> MAANEGNQPIPPEEEKEISSLLESIKIGKTSLKYRCFYLYDDKMTDLTEEQKETLKKLKLYQKEYYDYESKFEYELFLLRQKYHDLYGPIYDKRREALVGNGEAKIGTPNLPEFWLRALRNNNTVSHVIEDHDEEILVYLNDIRCDYIKKNKEKKEGFILSFYFATNPFFSNSVLTKTYHMKCVDCDNEPVLLHTEATVIDWYDNKNILKKNVVKKQHNKNSREVKTVQQTVNRDSFFHFFTSHKVPNSNVIKQLSKHEVAQLEMIIEGDYEVALTIKERIIPYAVDYYLGIIIESESNSIVSDVDSSYSSSENNSNYNSYESNNSAYNDENSNVDTNEYDDNEEEEEGAK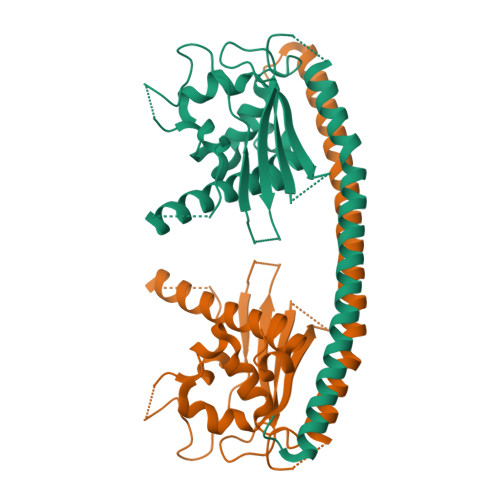SNEDPLTS>MKDVSKNQEENISDTALTNELIHLLGHSRHDWMNKLQLIKGNLSLQKYDRVFEMIEEMVIDAKHESKLSNLKTPHLAFDFLTFNWKTHYMTLEYEVLGEIKDLSAYDQKLAKLMRKLFHLFDQAVSRESENHLTVSLQTDHPDRQLILYLDFHGAFADPSAFDDIRQNGYEDVDIMRFEITSHECLIEIGL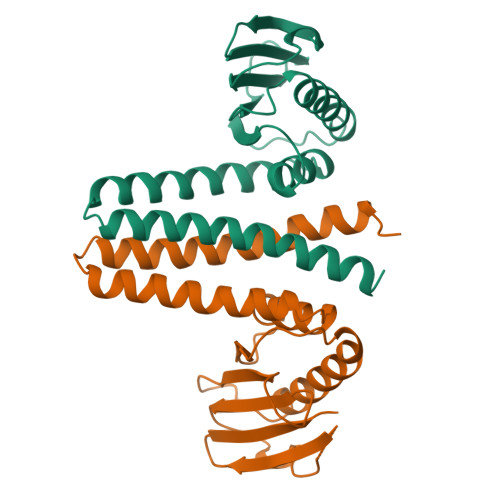D[2x]>MADVPAGVTLAEKQTLVRNNGSEVQSLDPHKIEGVPESNISRDLFEGLLVSDLDGHPAPGVAESWDNKDAKVWTFHLRKDAKWSDGTPVTAQDFVYSWQRSVDPNTASPYASYLQYGHIAGIDEILEGKKPITDLGVKAIDDHTLEVTLSEPVPYFYKLLVHPSTSPVPKAAIEKFGEKWTQPGNIVTNGAYTLKDWVVNERIVLERSPTYWNNAKTVINQVTYLPIASEVTDVNRYRSGEIDMTNNSMPIELFQKLKKEIPDEVHVDPYLCTYYYEINNQKPPFNDVRVRTALKLGMDRDIIVNKVKAQGNMPAYGYTPPYTDGAKLTQPEWFGWSQEKRNEEAKKLLAEAGYTADKPLTINLLYNTSDLHKKLAIAASSLWKKNIGVNVKLVNQEWKTFLDTRHQGTFDVARAGWCADYNEPTSFLNTMLSNSSMNTAHYKSPAFDSIMAETLKVTDEAQRTALYTKAEQQLDKDSAIVPVYYYVNARLVKPWVG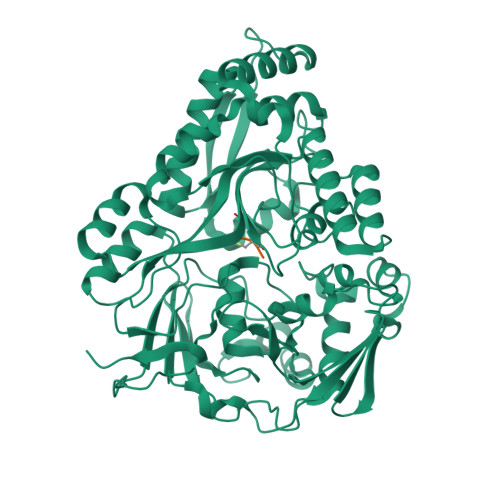GYTGKDPLDNTYTRNMYIVKHHHHHHH[8x];>[8x]KGE>HHHHHHMSGWVTVAGLGPGREDLVTPEVTAALAEATDIVGYIPYVARIAPREGLTLHPTDNRVELDRATHALEMAAEGRRVVVVSSGDPGVFAMASALFEALEAHPEHAGTEIRILPGITAMLAAAAAAGAPLGHDFCAINLSDNLKPFEILEKRLRHAARGDFAMAFYNPRSKSRPHQFTRVLEILREECEPGRLILFARAVTT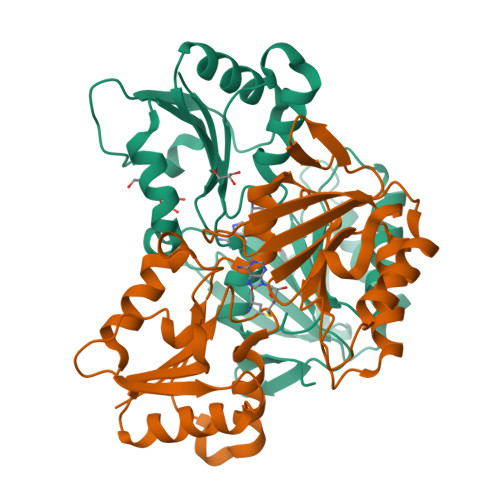PEQAISVVELRDATPEMADMRTVVLVGNAATRRVGPWVYTPRGVAP[4x]> DANLLNDRVLRAMLKA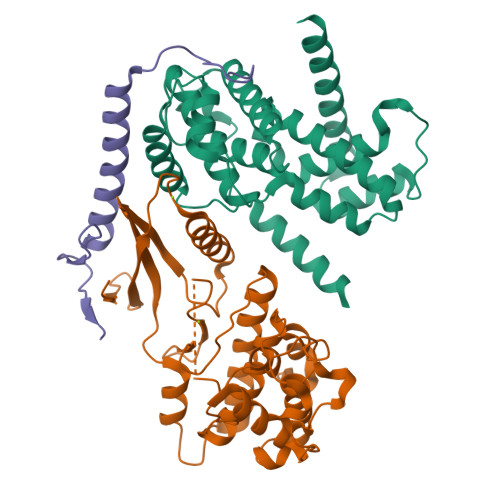EETCAPSVSYFKCVQKEVLPSMRKIVATWMLEVCEEQKCEEEVFPLAMNYLDRFLSLEPVKKSRLQLLGATCMFVASKMKETIPLTAEKLCIYTDNSIRPEELLQMELLLVNKLKWNLAAMTPHDFIEHFLSKMPEAEENKQIIRKHAQTFVALCATDVKFISNPPSMVAAGSVVAAVQGLNLRSPNNFLSYYRLTRFLSRVIKCDPDCLRACQEQIEALLESSLRQAQQNMD;> GEFATSRYEPVAEIGVGAYGTVYKARDPHSGHFVALKSVRVPNGEEGLPISTVREVALLRRLEAFEHPNVVRLMDVCATSRTDREIKVTLVFEHVDQDLRTYLDKAPPPGLPAETIKDLMRQFLRGLDFLHANCIVHRDLKPENILVTSGGTVKLADFGLARIYSYQMALTPVVVTLWYRAPEVLLQSTYATPVDMWSVGCIFAEMFRRKPLFCGNSEADQLGKIFDLIGLPPEDDWPRDVSLPRGAFPPRGPRPVQSVVPEMEESGAQLLLEMLTFNPHKRISAFRALQHSYLHKDEGNPE;> GEFKPSACRNLFGPVDHEELTRDLEKHCRDMEEASQRKWNFDFQNHKPLEGKYEWQEVEKGSLPEFYYRPPR> QKTGTAEMSSILEERILGADTSVDLEETGRVLSIGDGIARVHGLRNVQAEEMVEFSSGLKGMSLNLEPDNVGVVVFGNDKLIKEGDIVKRTGAIVDVPVGDELLGRVVDALGNAIDGKGPVGSKIRRRVGLKAPGIIPRISVREPMQTGIKAVDSLVPIGRGQRELIIGDRQTGKTSIAIDTIINQKRFNDGTDEKKKLYCIYVAIGQKRSTVAQLVKRLTDADAMKYTIVVSAT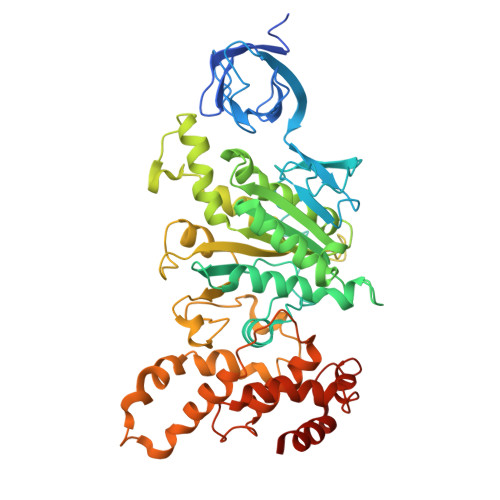ASDAAPLQYLAPYSGCSMGEYFRDNGKHALIIYDDLSKQAVAYRQMSLLLRRPPGREAYPGDVFYLHSRLLERAAKMNDSFGGGSLTALPVIETQAGDVSAYIPTNVISITDGQIFLETELFYKGIRPAINVGLSVSRVGSAAQTRAMKQVAGTMKLELAQYREVAAFAQFGSDLDAATQQLLSRGVRLTELLKQGQYSPMAIEEQVAVIYAGVRGYLDKLEPSKITKFESAFLSHVVSQHQSLLGNIRSDGKISEQSDAKLKEIVTNFLAGFEP> GATGRTTIAIDPVTRIEGHLKAEVVVENGKVVDARLSGGMYRGFETILRGRDPRDASQIVQRICGVCPTAHSTASVLALDEAFGAKVPNNGRITRNLIFGANYLQSHILHFYHLSAQDFVQGPDTAPFVPRFPKSDLRLSKELNKAGVDQYIEALEVRRICHEMVALFGGRMPHVQGQVVGGATEIPTKEKLVEYAARFKKVRDFVEQKYVPVVYTIGSKYKDMFKVGQGFKAALCVGAFPLDNSGKKHLFMPGVYAKGKDMPFDPSKIKEYVKYSWFAEETTGLNYKEGKTIPAPDKAGAYSFVKAPRYDGLSLEVGPLARMWVNNPELSPVGKKLLKDLFGISAKKFRDLGE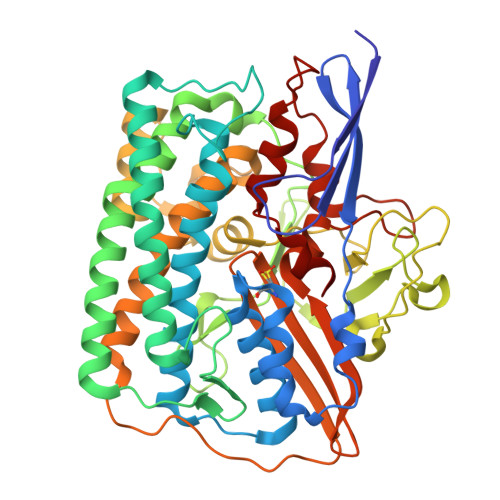EAAFSLMGRHVARAEETYYMLGAIEGWLKEIKAGEDTVVMPAVPASAEGTGFTEAPRGSLLHYVKVKDSKIDNYQIVSASLWNCNPRDDMGQRGAVEEALIGIPVDDIQNPVNVARLIRAFDPULACAVH>MPERLQVYKCEVCGNIVEVLNGGIGELVCCNQDMKLMSENTVDAAKEKHVPVIEKIDGGYKVKVGAVAHPMEEKHYIQWIELLADDKCYTQFL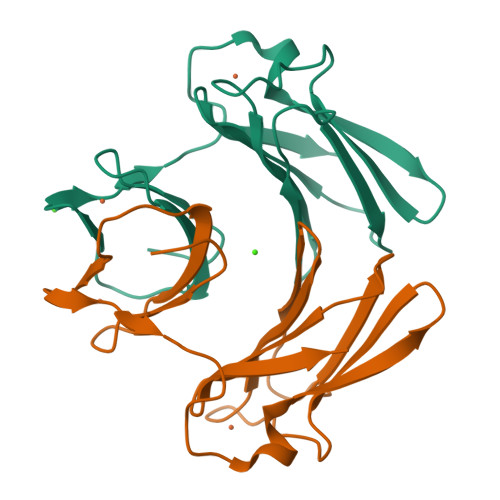KPGQAPEAVFLIEAAKVVAREYCNIHGHWKAEN[4x]> MAETKIVVGPQPFSVGEEYPWLAERDEDGAVVTFTGKVRNHNLGDSVNALTLEHYPGMTEKALAEIVDEARNRWPLGRVTVIHRIGELWPGDEIVFVG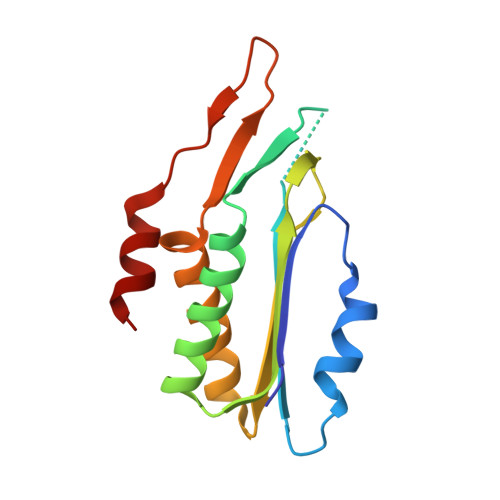VTSAHRSSAFEAGQFIMDYLKTRAPFWKREATPEGDRWVEARESDQQAAKRW>GMSTPSPALFFNTVNAYQRSAAIKAAVELNVFTAISQGIESSQSLAQKCQTSERGMRMLCDYLVIIGFMTKQAEGYRLTSDSAMFLDRQSKFYVGDAIEFLLSPMITNGFNDLTAAVLKGGTAISSEGTLSPEHPVWVQFAKAMSPMMANPAQLIAQLVNENKIEPLKVLDISA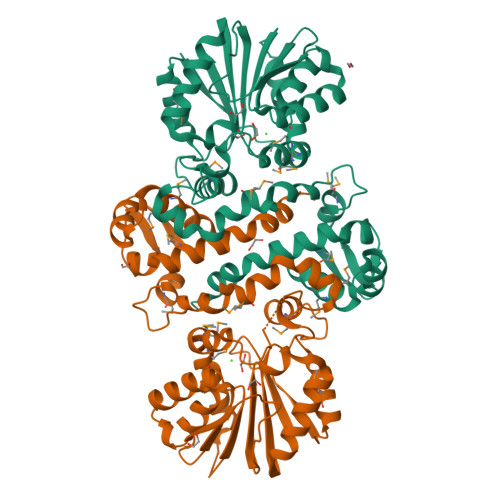SHGLFGIAVAQHNPNAEIFGVDWASVLEVAKENARIQGVASRYHTIAGSAFEVDYGNDYDLVLLPNFLHHFDVATCEQLLRKIKTALAVEGKVIVFDFIPNSDRITPPDAAAFSLVMLATTPNGDAYTFAEYESMFSNAGFSHSQLHSLPTTQQQVIVAYK[2x]>MIRNFHSLVKRVPRLALTPFFGFRTSMTLADKKLSTGEASVVLAEKIKGITQQNDITEYGTVISIGDGIARVFGLTKVQAGEMVEFKSGIRGMALNLETDNVGVVVLGNDRDIKEGDVVKRTGAIVDVPIGEAMCGRVFDALGNPIDGLGPLKTTQRARVEIKAPGIIPRQSVRQPMQTGIKCVDSLVPIGRGQRELIIGDRQTGKTAIAIDTILNQKEAFNTGDVKKQLYCIYVAVGQKRSTIANLVSILKQHDCMKFTIVVCATASDAAPLQFLAPYSGCAIGEFFRDNGKHALIIYDDLSKQAVAYRQMSLLLRRPPGREAYPGDVFYLHSRLLERAAKMNDSLGGGSLTALPVIETQAGDVSAYIPTNVISITDGQIFLETELFYKGIRPAINVGLSVSRVGSAAQIKAMKKIAGNLKLTLATYRELAAFSQFGSDLDAKTQQQLNTGERLVEMLKQNQYTPMKVEEQVCIIFAGVKGFLDALVTSEVLKFEKKFLEHVRTNHSALLKRIRDSGDLSEVDTNELNTIIPLFIQEGGFKLKAQ[3x];>MLSKALQRGIARAFSTTAKKEAPKTVKANGQVSQVIGAVVDVQFEGELPQILNALEVQGTQHRLVLEVAQHLGDSRVRTIAMDSTEGLVRGQPVVDTGLPISVPVGPGTLGRIMNVIGEPIDQRGPIKAAKLYPIHRDAPSFTDQATSAEILVTGIKVVDLLAPYARGGKIGLFGGAGVGKTVLIQELINNVAKHHGGYSVFAGVGERTREGNDLYHEMMDSKVISVKEGESRCALIFGQMNEPPGARARVGLTGLTVAEYFRDEEGKDVLLFVDNIFRFTQACSEVSALLGRIPSAVGYQPTLATDLGALQERITTTQKGSITSVQAIYVPADDLTDPAPATTFAHLDATTVLNRGLTELGIYPAVDPLDSTSRMLDPITIGEEHYTVARGVQKLLQDYKSLQDIIAILGVDDLSEEDKLVVARARKVQKFLSQPFFMSEVFSGIPGRFVNLKQNIASFKALLEGAGDEYPESCFYMKGDLEESLAAGRADALKSK[3x];> MQVIRKHLAQKGLFNPFLFNRFSTQQDITSVPGDKPPAIEDSIHGKYAGVLFSSASSNKSLNKVAEDMKYFNQLYKESEVFKSFLNNVSLKRNQQRDIISALGKTNFNPATNNLLETLIENKRLDSLPKIAEKYMDYYRILNKQESITIISAQELTAAEKQKVEQGLKKGNANVQFTVVYQVDPAILGGLQMYSGNNFLDCSLLSRVNKLKTEIAKISF;> MHSTLRVFTKNNCLSFTNMNRFSTAAQVAQANYSKFRADYSASVAAFQQRIKTIEKENTGSMKKPMAKAYEHPYNSEHHPLNFSAVKIAETFHDFIGPEQVSPHYESFAMSRKFLLTFWGGFFVLNFGMATVDLNWIMKSTYIPWIFWFQLMYFYVEGKNSMFMPLLQRFYRRAAANEIFTMEAFYHENIENKLRNLMRITKGQLEYWDIHTSYGEIRADSINNFLANEYLRLQSHITSRALNILKQAQAYETMNQAALLQKLIDDATSAIDNALKGDKKAEVLARSLDSAIDGLSKGYMDYQNDPLLPLILSSIEANVKKITTLSAQEQANLIGLTAEQLKSIKENDVRARKEFLESQPKLDNNLKNIESVKKILATWGK;> MSMLAKIAKNVVKTQALKNTTAAQTPSFQAPGNQDKILKWISTLSNKATTGESRSYCTQLSSLVSFYNKQHVEQIPTIDFNEWKSVISTQGLVDKVKENYESLIKEQYNTDAISKQISSASSKALDDIENELSFHAAIWLNAYADYTMFLFELEEYNDPNDYLMHENFDFFRGLETELEELTETHNYIPGAKDDVNLRGYLATQFAWGKKVISFYRHPADDFKCAKATKNMLGR;> MFGLASKGFINTSLVMVPQMNFGANLKQLKIRMKAIGSIKKITKAMKMVAASKMKAETSRLENGRNFAVGSVQKMLENESYVQKKKSTTAPKSTLLVPITSDKGLCGSVNSSIVREVKRLALNNRSAFGLLPVGEKGSSGLSRPFPDLLKSSIVNIQNVNFPTAAAIAHQVSTQGAGYDQVTLIYNHFKNAISYVVKHQELLPRAQFLNLFKYVTRHEAVEPELEYSKNYFFELYMASSVYNALLNSSASEQASRMNAMENASKNAGEILSKLTLDYNKARQAKITMELIEIISGASIV;> MNRSVNIAKNLIQTYRAMSVQSRFAFSTREEEWLDKRTKSQEKVYFDQEDRKAMKRLLEKLNTTSKFVEDSEYLAPQNLEVENILKRYHINYTQALIDELVDWKTGKN;> MNSLSSKKANSLVFKSIRNFTLQWGSLAERPMVDRVMSTSTWPVPYYQRLFKAYPIREKKDKMSLLLSDIDIDDTNWYQAKDFLRGSFRGRQIVDYVENNIASNTYILIQQDVANMAKAYVHDICGYIDVANKENVRILSKGDLI

The F-type ATP synthase (F1Fo-ATP synthase) is responsible for generating most of the cellular adenosine triphosphate (ATP) from adenosine diphosphate (ADP) and inorganic phosphate through rotary catalysis. In eukaryotes, ATP synthases are found in the inner mitochondrial membrane. The type III ATP synthase was detected in ciliates where it induces tubulation of the cristae membranes. In this study, we present the cryo-EM structures of the type III ATP synthase dimer and tetramer with associated lipids from the model organism Tetrahymena thermophila in complex with the natural inhibitor IF1.

Using masked refinements, the resolution of different regions reached 2.5–3.1 Å, allowing de novo modelling. Two copies of the ATP synthase dimer model were refined into the Fo-tetramer map generating a composite ATP synthase tetramer model. Both monomers are inhibited in the same rotary state by the natural inhibitor IF1. In our structure, the canonical inhibitory helix of IF1 is bound to the βDP-subunit of the F1-subcomplex. It is connected to the C-terminus dimerization domain through a flexible (unmodeled) linker. Subunit-b contributes its N-terminal helix to the peripheral stalk structure, in addition to the canonical C-terminal helix.> MNVEKFEGAELHVHVTGSISAALVPWWIHWLREFQPELVVNVSVTPAASRFLAVRALRHLANGKVWVDSWDDPDVPPEVNSGKSGASECFLVFPATLDTVMRLAQGRADSPALMMLQLTDAPLVIADTFPGSNEIVENNVQTLKLRPNVEFAPRVNGVRA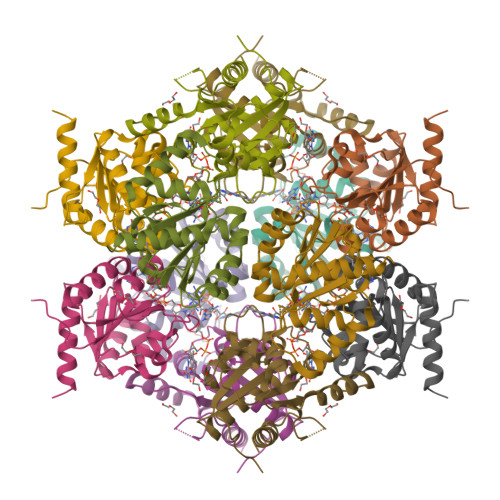SNRQTAEVGFNLPGALAAANRMRKEGRSGE> CGCAAAAAA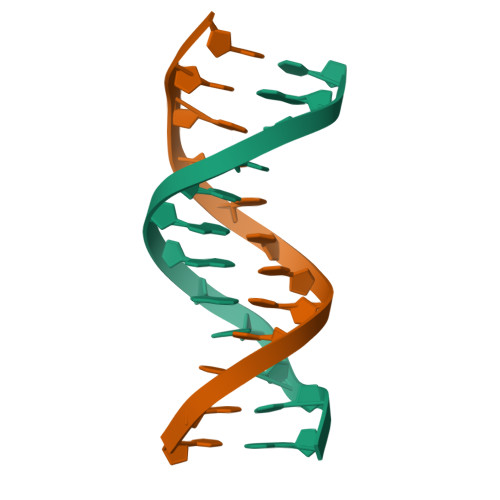GCG;> CGCTTTTTTGCG> FNEFKTPQID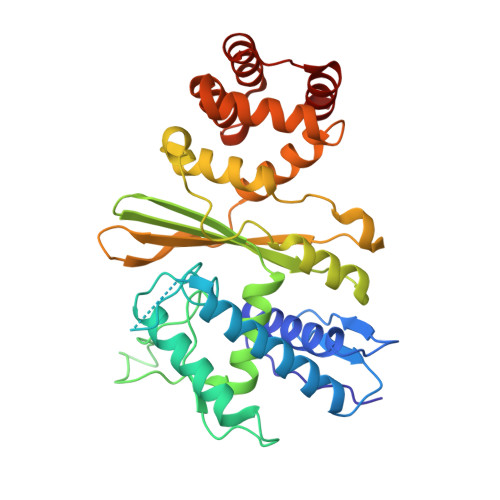PIFDLYVAYGYVVSLIRGGAKEATLIPHGASYLIQTDVSNEEFRHGLVDALSSMLSLHIALARHSPREGGKLVSDADFSAGANINNVYWDSVPRNLEKLMKDLEKKRSVKGTATIPITLMPSAGKYMLKHFGVQGGNPIKVDLLNYALAWVGFHYYTPYIKYAKGDTTWIHIYQIAPVEEVDMISILSLKDLKMHLPHYYESNLDFLINRRLALLYHLLHSEALELFTEKEFVIHSYTLERSGNNQAIRSFEEEEIGKLMDFLWKLKRRDFYHAIKFIDDLLKKATEGALALIDAIMNERLEGFYTALKLGKKAGVVSSREIVAALEDIIC>[2x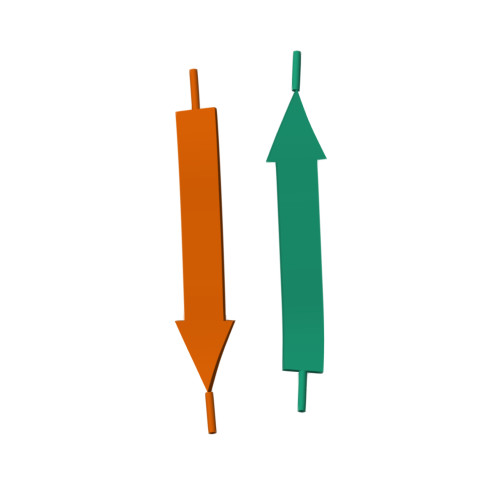]XEFIAWL> YSIEVRTHSALHVVKGAVVKAAGSAAKWTTSTYVKGNKGVLIVKAALELDKWAWAAMEALANEKVKENAPIKIYELPREEAEKMFGEDMYDLF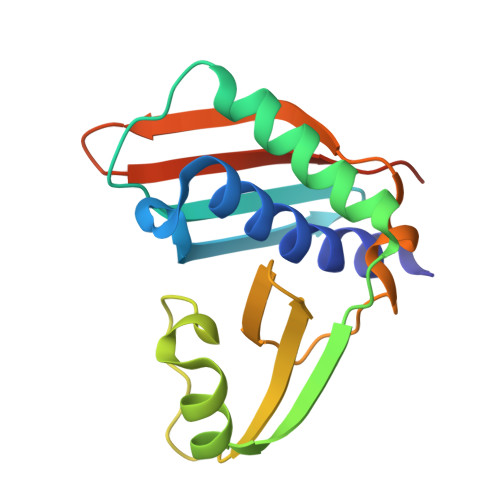PVPEDVRILKVVVIEDWNVNACNKEHTKTTGEIGPIKIRKVRFRKSKGLLEIHFELLELEHHHHHH Phytochromes (PHYs) are red-light sensing enzymatic switches first discovered in plants, with homologs in the photosynthetic and nonphotosynthetic bacteria. PHYs are composed of a photosensory core module (PCM) and an effector, enzymatic domain. In bacteriophytochromes (BphPs), the PCM consists of three domains named PAS (Per ARNT Sim), GAF (cGMP phosphodiesterase/adenylyl cyclase/FhIA), and PHY (phytochrome-specific GAF-related) [Fig. 1(a)].1–5 The effector domain is typically a histidine kinase, covalently linked to a PHY domain, although other nonenzymatic output domains can be found. However, both proteins bind the same bilin chromophore and share a large amino acid sequence identity (38%).5,14,18 Biliverdin (BV) is an open-chain tetrapyrrole that is highly conjugated and allows for reversible photoconversion in BphPs between the red light absorbing (Pr, λmax 700 nm) and far-red light absorbing (Pfr, λmax 750 nm) states. Here, we report three crystal structures of the SaBphP2 photosensory core module (PCM), lacking the effector histidine kinase domain.

The reported structures are of a SaBphP2 PCM in the wild-type (wt) and mutant forms determined at 1.65 Å and 2.2 Å, respectively. This is the highest resolution structure of any PCM construct in the wild-type form to date, revealing the important intricate details of the hydrogen-bonding network of the conserved amino acids and waters stabilizing BV chromophore in the Pr state. The wild-type protein crystallized in the dark in the Pr state in space group P21. Crystals grown from the PCM constructs diffracted to 1.65 Å resolution at 100 K and 2.1 Å at 293 K. Given the high resolution of SaBphP2 wild-type structure, we clearly observe an intricate network of waters and conserved amino acids which stabilize the BV-chromophore in the Pr state. This network includes residues from including the PASDIP motif in the GAF domain and the PRXSF motif of the PHY domain [Figs. 2(c) and 3(d)]. Interestingly, not a single amino acid from the PHY domain forms direct contact with the BV chromophore. Crystal structures of the wild-type classical SaBphP2 determined at the highest resolution of any PCM to date reveal an intricate network of hydrogen bonds between conserved amino acids, neighboring water molecules, and BV which all stabilize the Pr state. To our surprise, the dimer interface structure of SaBphP2 is different from those of the related classical phytochromes such as DrBphP21,50 and RpBphP2.8 They all have an extensive helical kink at the dimer interface that is absent from SaBphP2. In the SaBphP2 PCM crystals, subunits A and B form a noncrystallographic dimer.

>[2x]DLSQCDREPIHLLGGIQSHGVLLAFRGPDRLLEVVSANAQALLGRPPETLLGQPVGRVLPAEVLAQWEPLVARGSVRVVLPAGAYRALLHESDGLTVLELEPAELQPGMEETALEVVRRLVSPLAGVKGTQALLQTAADTVRALTGFDRVMVYRFDADWHGEVLAESKRGGMDGFLGMHFPATDIPVQARALYTRNPLRLIADARARPVPLLPPVVPALGRPLDLSNSALRSVSPVHLEYLRNMGVGASFSLSLLKEGVLWGLIACHHLEPLHISHERRRACEVLTQLLALQLSAEERAAEASEDAHRAALLGQLATAMGEGGTLEEVLEKESERVLALTGAAGVALLLGEEPLLVGCTPAQDEVEALVAWLATQPFQTSFHTDRLGTVYPPLAARADVAAGILAVRLAPAAARFAIWFRPEVARTISWAGNPRKPAEPEPGHQRLHPRGSFQAWEETVRDTSLPWKRADLGAAEGFRGAL> MPRVVPDQ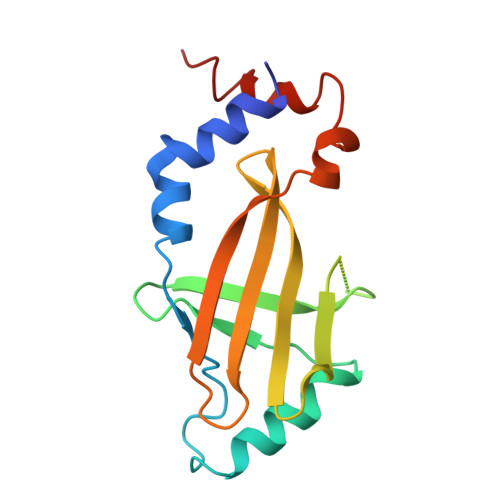RSKFENEEFFRKLSRECEIKYTGFRDRPHEERQARFQNACRDGRSEIAFVATGTNLSLQFFPASWQGEQRQTPSREYVDLEREAGKVYLKAPMILNGVCVIWKGWIDLQRLDGMGCLEFDEERAQQEDALAQQAFEEARRRTR> AANDNNVEWNGLFHDQGPLFDNAPEPTSTQSVTLKLRTFKGDITSANIKYWDTADNAFHWVPMVWDSNDPTGTFDYWKGTIPASPSIKYYRFQINDGTSTAWYNGNGPSSTEPNADDFYIIPNFKTPDWLKNGVMYQIFPDRFYNGDSSNDVQTGSYTYNGTPTEKKAWGSSVYADPGYDNSLVFFGGDLAGIDQKLGYIKKTLGANILYLNPIFKAPTNHKYDTQDYMAVDPAFGDNSTLQTLINDIHSTANGPKGYLILDGVFNHTGDSHPWFDKYNNFSSQGAYESQSSPWYNYYTFYTWPDSYASFLGFNSLPKLNYGNSGSAVRGVIYNNSNSVAKTYLNPPYSVDGWRLNAAQYVDANGNNGSDVTNHQIWSEFRNAVKGVNSNAAIIGEYWGNANPWTAQGNQWDAATNFDGFTQPVSEWITGKDYQNNSASISTTQFDSWLRGTRANYPTNVQQSMMNFLSNHDITRFATRSGGDLWKTYLALIFQMTYVGTPTIYYGDEYGMQGGADPDNRRSFDWSQATPSNSAVALTQKLITIRNQYPALRTGSFMTLITDDTNKIYSYGRFDNVNRIAVVLNNDSVSHTVNVPVWQLSMPNGSTVT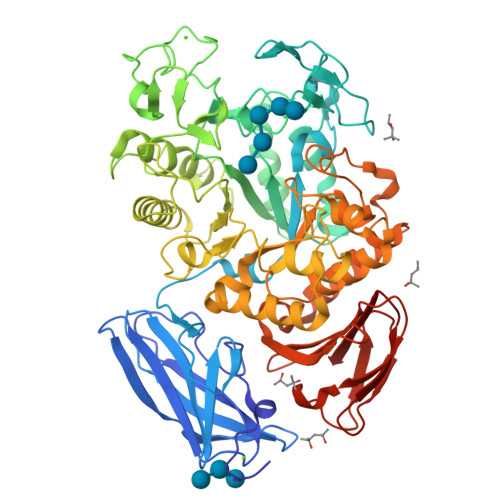DKITGHSYTVQNGMVTVAVDGHYGAVLAQ>MAFPIPARQLFIDGEWREPIKKNRIPVINPSTEEIIGDIPAATAEDVEVAVVAARRAFRRNNWSATSGAHRATYLRAIAAKITEKKDHFVKLETIDSGKPFDEAVLDIDDVASCFEYFAGQAEALDGKQKAPVTLPMERFKSHVLRQPLGVVGLISPWNYPLLMATWKIAPALAAGCTAVLKPSELASVTCLEFGEVCNEVGLPPGVLNILTGLGPDAGAPLVSHPDVDKIAFTGSSATGSKVMASAAQLVKPVTLELGGKSPIVVFEDVDIDKVVEWTIFGCFWTNGQICSATSRLLVHESIAAEFVDKLVKWTKNIKISDPFEEGCRLGPVISKGQYDKIMKFISTAKSEGATILYGGSRPEHLKKGYYIEPTIVTDISTS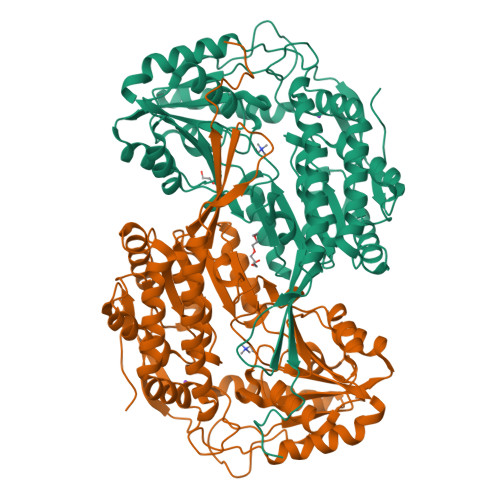MQIWKEEVFGPVLCVKTFSSEDEAIALANDTEYGLAAAVFSNDLERCERITKALEVGAVWVNCSQPCFVQAPWGGIKRSGFGRELGEWGIQNYLNIKQVTQDISDEPWGWYKSP[4x]>[2x]MSQSNRELVVDFLSYKLSQKGYSWSQPMAAVKQALR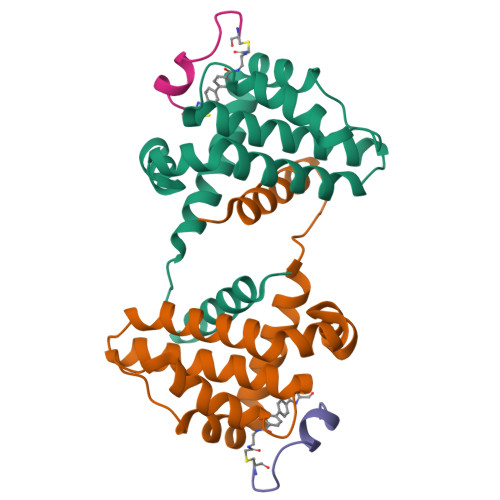EAGDEFELRYRRAFSDLTSQLHITPGTAYQSFEQVVNELFRDGVNWGRIVAFFSFGGALCVESVDKEMQVLVSRIAAWMATYLNDHLEPWIQENGGWDTFVELYG;>[2x]TPEWASTLRPECXXP> MNPNFTTEHTWQGRHDPEDGQAGRRVHHIACPIQVGELANQEPGVALIGFECDAGVERNKGRTGAKHAPSLIKQALANLAWHHPIPIYDLGNIRCEGDELEQAQQECAQ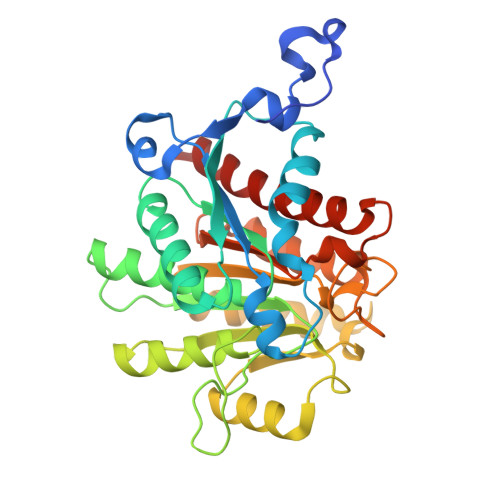VIQQALPHARAIVLGGGHEIAWATFQGLAQHFLATGVKQPRIGIINFDAHFDLRTFESELAPVRPSSGTPFNQIHHFCQQQGWDFHYACLGVSRASNTPALFERADKLGVWYVEDKAFSPLSLKDHLTQLQHFIDDCDYLYLTIDLDVFPAASAPGVSAPAARGVSLEALAPYFDRILHYKNKLMIADIAEYNPSFDIDQHTARLAARLCWDIANAMAEQVQSIRHP> MIIDSQSVVQYTFKIDILEKLYKFLPNLYHSIVNELVEELHLENNDFLIGTYKDL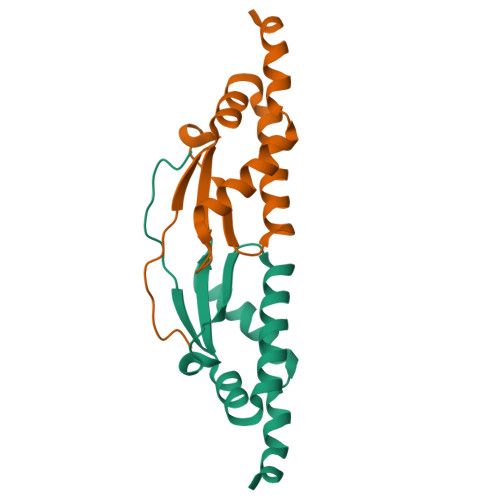SKAGYFYVIPAPGKNIDDVLKTIMIYVHDYEIEDYFELEHHHHHH>[2x]GGSHTADRWRVSL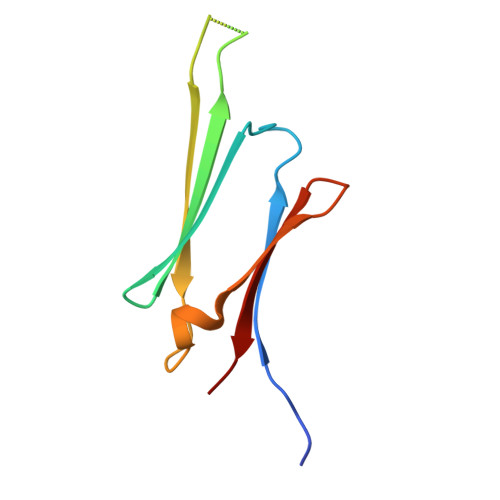DVNHFAPDELTVKTKDGVVEITGKHAARQDEHGYISRCFTRKYTLPPGVDPTQVSSSLSPEGTLTVEAPMPK Whereas yeasts only have one Aurora kinase, metazoans generally have two, named Aurora A and B. Mammals, but not other vertebrates, also have a third family member, Aurora C. Aurora A localizes to centrosomes and spindle microtubules and plays important roles in centrosome maturation, controlling spindle length and bipolarity, asymmetric cell division, and promoting mitotic entry both in unperturbed cells and following DNA damage. Aurora A has multiple regulators, with the best-studied one being TPX2, which activates the kinase and targets it to spindle microtubules. As in the case of Aurora B, phosphorylation of this threonine [which readily occurs in vitro even in the absence of TPX2 or other activators (16)] promotes high levels of kinase activity. The Aurora kinases therefore emerged as attractive drug targets in cancer and became the focus of intense drug discovery efforts.

To gain insight into the remarkable biochemical potency and Aurora A-selective nature of the MK-8745/MK-5108 class of compounds, we determined the 2.2 Å X-ray crystal structure of the human Aurora A kinase domain bound to MK-5108. In the inhibitor complex, the Aurora A kinase domain adopts an inactive conformation in which both the αC helix (orange) and particularly the activation loop (yellow) are improperly positioned for catalysis (Figure 9B – compare MK-5108-bound versus ADP-bound structures). Electron density maps indicate that both Thr 287 (which adopts two alternate conformations; only one is illustrated) and Thr 288 are phosphorylated, showing that the inhibitor is able to interact with the activated form of the enzyme. Consistent with its action as an ATP-competitive inhibitor, MK-5108 inserts itself into the nucleotide-binding pocket between the two lobes of the kinase in the same orientation as its parent compound VX-680. The picomolar affinity of MK-5108 for Aurora A is explained by the extensive polar and van der Waals interactions it forms with 22 residues throughout the active site. The 2-fluoro, 3-chlorophenol on the opposite end of the inhibitor packs against the side chains of the catalytic lysine (Lys 162), precluding its active conformation, as well as against Phe 275 of the DFG motif. This interaction stabilizes a flipped, inactive conformation of the DFG motif that is intermediate between the active “DFG-in” state (Figure 9B – ADP-bound) and the canonical “DFG-out” conformation. Importantly, the 2-fluoro, 3-chlorophenol moiety of MK-5108 forms a likely highly energetically favorable edge-face aromatic pi stacking interaction with the indole of Trp 277. The interaction between MK-5108 and the side chain of Trp 277 has the effect of “pinning down” the activation loop at its N-terminal end and disfavors its adoption of an active conformation.

> GPGSKKRQWALEDFEIGRPLGKGKFGNVYLAREKQSKFILALKVLFKAQLEKAGVEHQLRREVEIQSHLRHPNILRLYGYFHDATRVYLILEYAPLGTVYRELQKLSKFDEQRTATYITELANALSYCHSKRVIHRDIKPENLLLGSAGELKIADFGWSVHAPSSRRTTLCGTLDYLPPEMIEGRMHDEKVDLWSLGVLCYEFLVGKPPFEANTYQETYKRISRVEFTFPDFVTEGARDLISRLLKHNPSQRPMLREVLEHPWITANSSKP>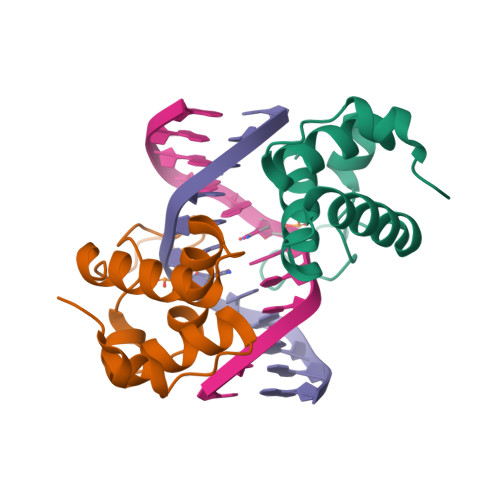[2x]GDEKQFQIEKWQIARCNKSKPQKFINDLMQVLYTNEYMATHSLTGAKSSTSRDKAVKPAMNQNEVQEIIGVTKQLFPNTDDVSIRRMIGQKLNNCTKKPNLSK>GSHMGANDADRPTNAESLDGIKSVIAGGVSSSMRAAAVPLPLVVRSAGGCLLRDVEDGEIIDLNMGYGPHLFGYADREVLDAVADQFAKGHMTGLPHELDARAGALIAELVPGVEQVRFANSGTEAVASALRLARATTGRTLVVTFEGHYHGWSETVLRAGKTALHMEGTRPTDVVPGALGMIPEALAHTVQLGWNDPDALRELFARDGDRIAAVIVEPVLANAGVIPPAPGFLQLLRELTGRSGAMLVFDEVITGFRVARGGAQERYGVEPDLTVLSRVMGGGFPVAAFGGRRHAMRMLASNEAHHAGVYAG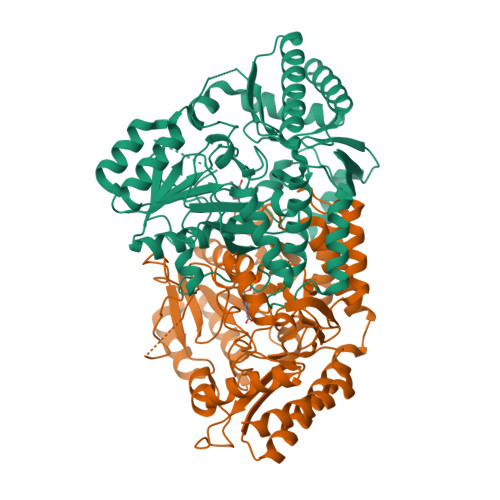NHAALRAVVAMLGKIRSLPDLYERLEDTGQYMEDTVREVFATEKRPVHINRVGTLMSVALLKGSAEPSAEPRDLRQLAALVDFPRHRRLQTLAQKEGVYFHPNALEPWFLSTAHTRDVIDKVAGALQRSLVGLG[6x]>GPLGSNKAQKNQSKRARSDALLWLAANFPEAFDNSLRIRPLKIGIMSDILQHAEKAEQVGVSKSKLREAVVLFTRRLDYLACLKAREVRIDLHGNPVAEVTEEEAENASMKIKKRVEK[10x]

The ProQ/FinO family of RNA binding proteins mediate sRNA-directed gene regulation throughout gram-negative bacteria. The RocC/RocR system regulates competence, a specialized physiological state involving the coordinated expression of multiple genes which allows the bacteria to uptake environmental DNA and integrate it into its chromosome (i.e., natural transformation). RocC binds and stabilizes RocR, which in turn binds and represses a series of mRNA targets that encode components of the DNA uptake system.

We crystallized and determined the structure of RocC both alone and in complex with RocRSL3 containing a modified stem-loop with a nine base-pair stem and a tetraloop (RocR9bp-tet) at 3.2 Å. The asymmetric unit contains six copies of apo-RocC14-126 and four copies of the protein–RNA complex. Overall, the hairpin-tail RNA binds to one side of the ProQ/FinO domain, largely through interactions between the protein and the RNA backbone. The hairpin portion of the RNA is bound by the N-terminal portion of α5 with supplementary interactions from α2. The N-terminus of this helix hydrogen bonds to all four non-bridging oxygens in two successive phosphate groups—C21 and C22. The 4-nucleotide single-stranded 3’ tail (5’-U25U26C27U28−3’) adopts a hook-like structure. The 3’ terminal nucleotide, U28 bends back such that its 3’-hydroxyl hydrogen bonds with the penultimate phosphate linking U26 and C27. The terminal U28 is bound within a well-conserved and structurally rigid pocket that is formed between α5 and a β-turn at the N-terminus of α4. The pocket contains Tyr87 and Arg97, which are both among the most highly conserved residues in the ProQ/FinO domain family and together recognize the phosphate of U28. However, how FinO could at once bind to a hairpin RNA while destabilizing its base pairing was unclear. The RocC/RocR structure reveals that RocC only binds the 3’ strand of the hairpin, leaving the 5’ side unencumbered so that it could be peeled away to allow duplexing with a complementary RNA.>[2x]GSPLTPRFTAEEKEV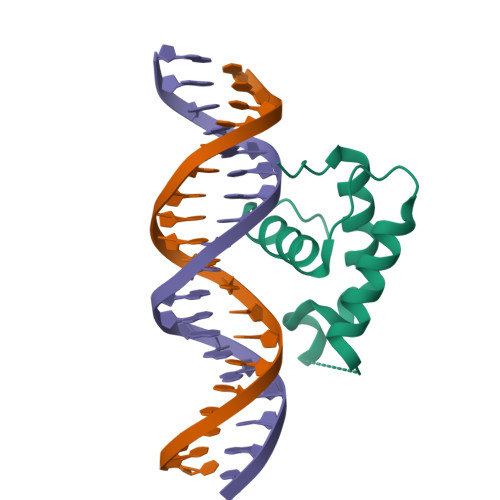LYTLFHLHEEVIDIKHRKKQRNKYSVRETWDKIVKDFNSHPHVSAMRNIKQIQKFWLNSRLRKQYPY>MRDPQKRNSHRIPATIPVEVANADGSIIVTGVTEDLSMGGAAVKMSWPAKLSGPTPVYIR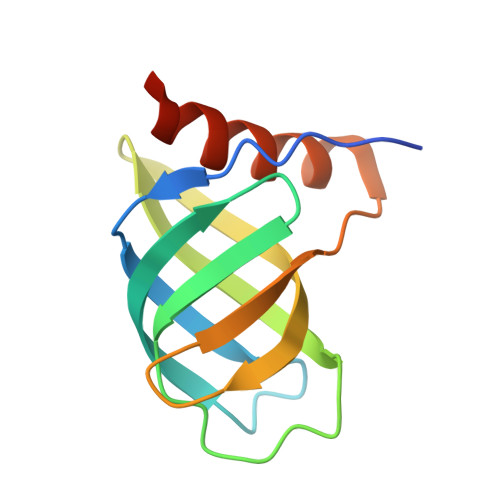TVLDGEELILPARIIRAGNGRGIFIWTIDNLQQEFSVIRLVFGLEHHHHHH[2x]>SNAMDTQTLNSDLRVFMHHIYEFEKGVRSMVLATLANDDIPYAEERLRSRQIPYFAQPTPNTERTNLFFG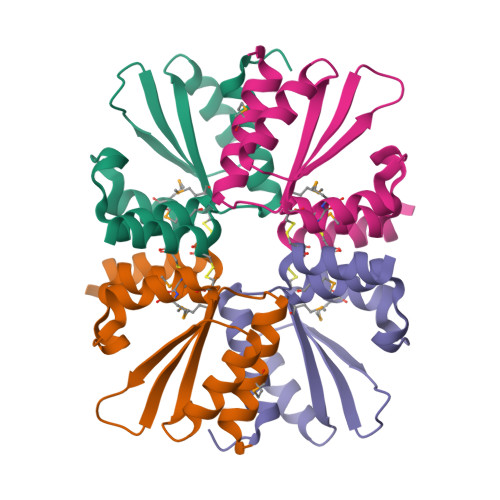CKECMEAIRLFVSGRSLNSLTPEEDFIIGAMLGYDICRQCERYCRRKSNS[2x]3-[8-azanyl-1-(4-ethoxy-8-fluoranyl-2-phenyl-quinolin-7-yl)imidazo[1,5-a]pyrazin-3-yl]-1-methyl-cyclobutan-1-ol | C28 H26 F N5 O2 | 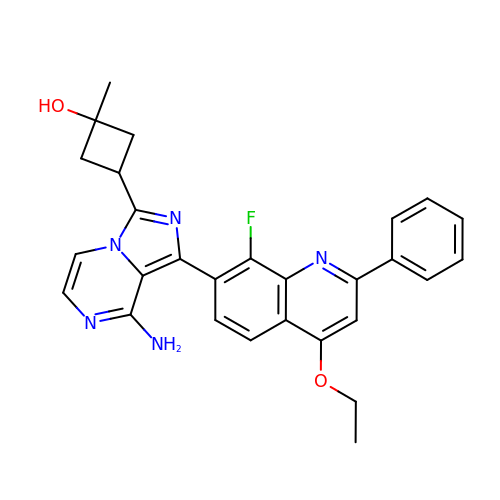TVXAIWDTRFFVCZ-OOTKOPMESA-N> 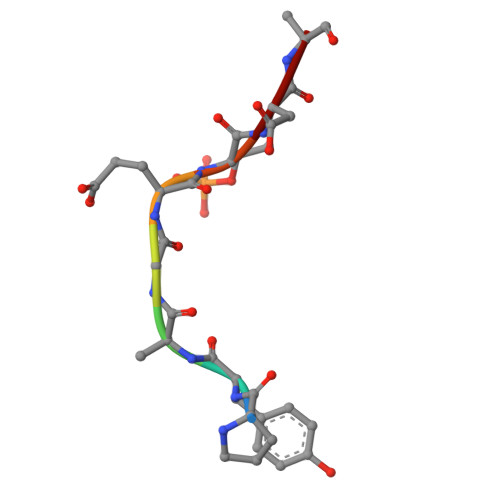PYAGETDE> EAISVPAPFTKVAPKGDRVLVKVAEEEVKTRGGILLPPSAIKKPTSGEVVQLGDGRVGDGEVRPFYLQPGQTVVYSKFGFMYQDLKLSNGEEYILIREDDVIGIMPRANAQADDVPELQPLADRVLIKVEEVADVTMGGVFLPETAKERPLSGTVVRVGPGKYDKDA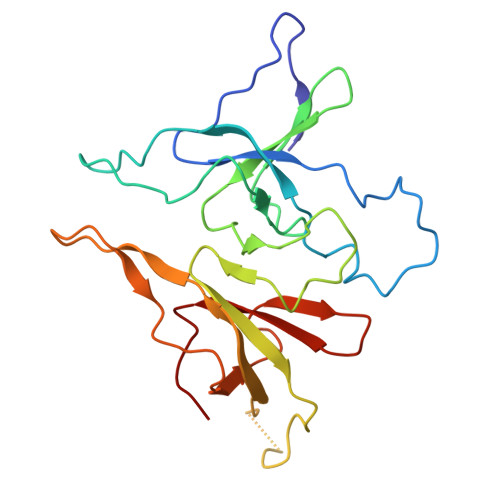EGKRRTVPLAPGDKVLYFKYAGDNMETPSGDKFVVLRSDDVLCKA>QDLMASGNTTVKATFGKDSSVVKWVVLAEVLVGAVMYMMTKNVKFLAGFAIISVFIAVGMAVVGL[75x];> MRAFSTLDRENETFVPSVRVYADGETEDNSFSLKYRSNWTPGRFNSTGAKTKQWHYPSPYSRGALSVTSIDQGAYKRSGSSWGRPYEEKAGFGFSLDARSCYSLFPVSQNLTYIEVPQNVANRASTEVLQKVTQGNFNLGVALAEARSTASQLATQTIALVKAYTAARRGNWRQALRYLALNEDRKFRSKHVAGRWLELQFGWLPLMSDIQGAYEMLTKVHLQEFLPMRAVRQVGTNIKLDGRLSYPAANFQTTCN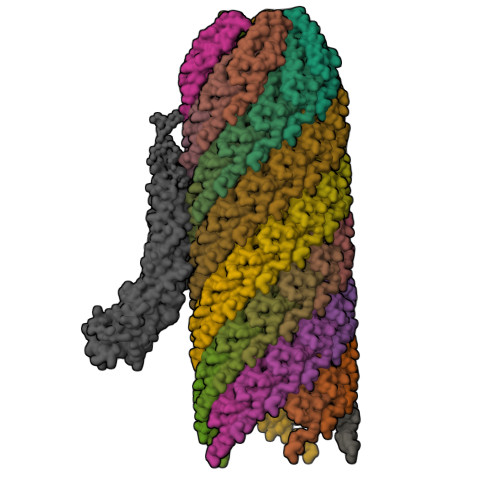ISRRIVIWFYINDARLAWLSSLGILNPLGIVWEKVPFSFVVDWLLPVGNMLEGLTAPVGCSYMSGTVTDVITGESIISVDAPYGWTVERQGTAKAQISAMHRGVQSVWPTTGAYVKSPFSMVHTLDALALIRQRLSR> MKEFYLTVEQIGDSIFERYIDSNGRERTREVEYKPSLFAHCPESQATKYFDIYGKPCTRKLFANMRDASQWIKRMEDIGLEALGMDDFK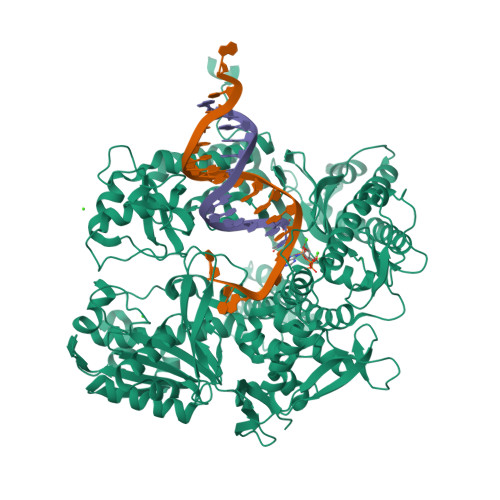LAYLSDTYNYEIKYDHTKIRVANFDIEVTSPDGFPEPSQAKHPIDAITHYDSIDDRFYVFDLLNSPYGNVEEWSIEIAAKLQEQGGDEVPSEIIDKIIYMPFDNEKELLMEYLNFWQQKTPVILTGWNVESFAIPYVYNRIKNIFGESTAKRLSPHRKTRVKVIENMYGSREIITLFGISVLDYIDLYKKFSFTNQPSYSLDYISEFELNVGKLKYDGPISKLRESNHQRYISYNIIAVYRVLQIDAKRQFINLSLDMGYYAKIQIQSVFSPIKTWDAIIFNSLKEQNKVIPQGRSHPVQPYPGAFVKEPIPNRYKYVMSFDLTSLYPSIIRQVNISPETIAGTFKVAPLHDYINAVAERPSDVYSCSPNGMMYYKDRDGVVPTEITKVFNQRKEHKGYMLAAQRNGEIIKEALHNPNLSVDEPLDVDYRFDFSDEIKEKIKKLSAKSLNEMLFRAQRTEVAGMTAQINRKLLINSLYGALGNVWFRYYDLRNATAITTFGQMALQWIERKVNEYLNEVCGTEGEAFVLYGDTDSIYVSADKIIDKVGESKFRDTNHWVDFLDKFARERMEPAIDRGFREMCEYMNNKQHLMFMDREAIAGPPLGSKGIGGFWTGKKRYALNVWDMEGTRYAEPKLKIMGLETQKSSTPKAVQKALKECIRRMLQEGEESLQEYFKEFEKEFRQLNYISIASVSSANNIAKYDVGGFPGPKCPFHIRGILTYNRAIKGNIDAPQVVEGEKVYVLPLREGNPFGDKCIAWPSGTEITDLIKDDVLHWMDYTVLLEKTFIKPLEGFTSAAKLDYEKKASLFDMFDF> MTAAAFDDLRPRLGRLTEETIDIAREVLVEGKSQSDVARERGLSRQRVSSMVKSVVSAANEIPREWQRVEVWLPPNLAEKVRQMEADAKADVARKNQLTDAALEHHHHHH

ArdK is a 102 amino acid protein encoded by the broad host range conjugative plasmid R388. In R388, ArdK represses the expression of five genes by its binding to their respective promoters (PardC, Porf7, Pssb, Porf12 and Porf14). The KorA family of transcriptional regulators includes plasmid-borne repressors involved in plasmid stability and conjugation. Our structural analyses show that ArdK, a member of this family, can form a symmetric dimer similar to that observed for KorA, yet it binds direct sequence repeats as a non-symmetric dimer.

ArdK was crystallized as described in the Materials and Methods, and resolved to 3.0 Å resolution. In the crystal of the apo structure, there is a single ArdK molecule in the asymmetric unit. This molecule contains an N-terminal HTH domain (residues 1–62) and a C-terminal domain with a C-terminal α-helix (residues 75–102) connected by a linker region (residues 63–74). The C-terminal domain forms a β-sheet with its symmetry-related molecule. Thus, the biological assembly is very probably a dimer containing two HTH domains (α1–α4) and a dimerization domain (DD, β1 and α5). In fact, according to S75 gel filtration data, the protein purified as a dimer in solution. The structure of the HTH and DD domains in ArdK is strikingly similar to the structure of these domains in KorA. Both the HTH and the DD of ArdK show a root mean square deviation (RMSD) of 0.83 Å and 1.35 Å with their respective homologue domains in KorA. Comparison between both structures revealed that both dimers are symmetrical, but the orientation of the HTH differs: in ArdK, the HTH domains are rotated 150° with respect to their position in KorA. As a consequence, the electropositive N-terminal ends of the recognition α4 helices point towards each other in KorA, whereas they are pointing in opposite directions in ArdK.Here we report cryo-electron microscopic structures of the heme translocation complex CcmABCD from E. coli, alone and bound to the heme chaperone CcmE. CcmABCD forms a heterooctameric complex centered around the ABC transporter CcmAB that does not by itself transport heme. Our data suggest that the complex flops a heme group from the inner to the outer leaflet at its CcmBC interfaces, driven by ATP hydrolysis at CcmA. A conserved heme-handling motif (WxWD) at the periplasmic side of CcmC rotates the heme by 90° for covalent attachment to the heme chaperone CcmE that we find interacting exclusively with the CcmB subunit.

In our cryo-EM single particle data of the native complex, the two most highly resolved 3D classes contained the Ccm(ABCD)2 complex, but one of these additionally featured a prominent periplasmic domain that after refinement was modeled as CcmE with its N-terminal transmembrane helix. This helix interacted exclusively with helix hVI of CcmB, with the periplasmic domain of CcmE poised above the CcmBC interface on one side of the complex. Although the observed interface was small, the interaction of CcmB with CcmE was well resolved in the maps. 29 % of all particles used for the final refinement contained CcmE, and although at lower contour levels a second copy of the chaperone on the opposite side of the complex was apparent and the N-terminal helix of CcmE was visible in lower-resolution reconstructions during data processing, the relevant class predominantly contained a single copy of CcmE, with slightly lower local resolution and presumably substoichiometric occupancy. The transmembrane helix of CcmE was modeled from residue N2 to S32 and is followed by a short, flexible hinge preceding the β-barrel domain that commences at F37. The heme-coordinating residues H130 and Y134 faced the membrane but were situated above CcmB rather than CcmC. The association of CcmE to the complex also did not seem to affect its structure, and there was no discernible change observed in CcmB. In the experimental structure, the periplasmic domain of CcmE showed enhanced mobility and a lower local resolution than the core complex, which in the absence of a bound heme group is not surprising. AlphaFold2 yielded a model of a symmetric Ccm(ABCDE)2 complex with a root-mean-squared deviation from the experimental structure of 3.1 Å for all atoms that also reproduced the observed association of CcmE to the heterooctameric core very well. However, the periplasmic domain of CcmE was rotated by about 90° towards CcmC, placing it above loop 5 and the WxWD motif of the latter.

>[2x]MASWSHPQFEKMGMLEARELLCERDERTLFSGLSFTLNAGEWVQITGSNGAGKTTLLRLLTGLSRPDAGEVLWQGQPLHQVRDSYHQNLLWIGHQPGIKTRLTALENLHFYHRDGDTAQCLEALAQAGLAGFEDIPVNQLSAGQQRRVALARLWLTRATLWILDEPFTAIDVNGVDRLTQRMAQHTEQGGIVILTTHQPLNVAESKIRRISLTQTRAA;>MMFWRIFRLELRVAFRHSAEIANPLWFFLIVITLFPLSIGPEPQLLARIAPGIIWVAALLSSLLALERLFRDDLQDGSLEQLMLLPLPLPAVVLAKVMAHWMVTGLPLLILSPLVAMLLGMDVYGWQVMALTLLLGTPTLGFLGAPGVALTVGLKRGGVLLSILVLPLTIPLLIFATAAMDAASMHLPVDGYLAILGALLAGTATLSPFATAAALRISIQ[2x];>MWKTLHQLAIPPRLYQICGWFIPWLAIASVVVLTVGWIWGFGFAPADYQQGNSYRIIYLHVPAAIWSMGIYASMAVAAFIGLVWQMKMANLAVAAMAPIGAVFTFIALVTGSAWGKPMWGTWWVWDARLTSELVLLFLYVGVIALWHAFDDRRLAGRAAGILVLIGVVNLPIIHYSVEWWNTLHQGSTRMQQSIDPAMRSPLRWSIFGFLLLSATLTLMRMRNLILLMEKRRPWVSELILKRGRK[2x];>MTPAFASWNEFFAMGGYAFFVWLAVVMTVIPLVVLVVHSVMQHRAILRGVAQQRAREARLRAAQQQEAA[2x];> MNIRRKNRLWIACAVLAGLALTIGLVLYALRSNIDLFYTPGEILYGKRETQQMPEVGQRLRVGGMVMPGSVQRDPNSLKVTFTIYDAEGSVDVSYEGILPDLFREGQGVVVQGELEKGNHILAKEVLAKHDENYTPPEVEKAMEANHRRPASVYKDPAS>MAMVNTTTRLSDDALAFLSERHLAMLTTLRADNSPHVVAVGFTFDPKTHIARVITTGGSQKAV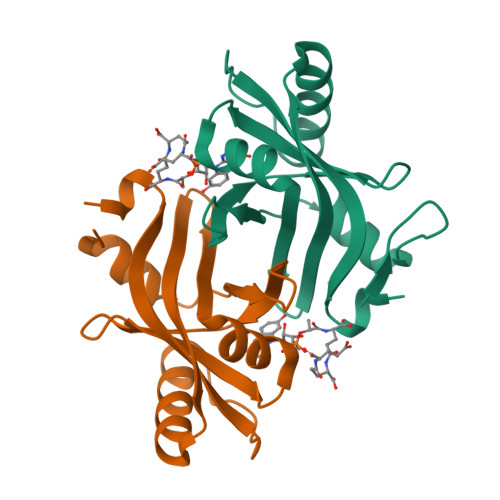NADRSGLAVLSQVDGARWLSLEGRAAVNSDIDAVRDAELRYAQRYRTPRPNPRRVVIEVQIERVLGSADLLD[4x]2-(6-methoxy-1-oxo-1,3-dihydro-2H-isoindol-2-yl)-N-[4-(piperazin-1-yl)pyridin-3-yl]-1,3-thiazole-4-carboxamide | C22 H22 N6 O3 S | 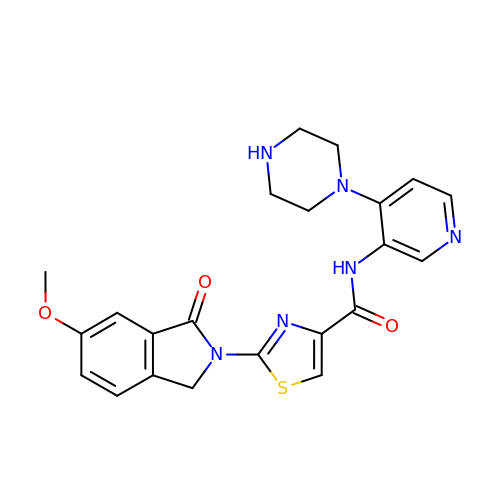KLJVDMAOKMSBQX-UHFFFAOYSA-N>GNSGRFERDAFDTLFDHAPDKLSVVKKSLITFVNKHLNKLNLEVTELETQFADGVY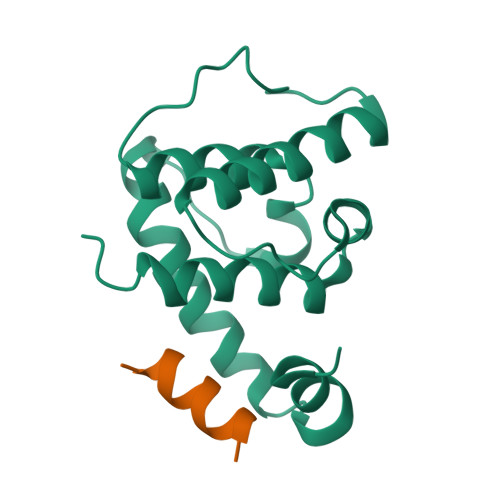LVLLMGLLEDYFVPLHHFYLTPESFDQKVHNVSFAFELMLDGGLKKPKARPEDVVNLDLKSTLRVLYNLFTKYKNVE[10x];>[7x]XMDDLDALLADLESTTSHISKX>GSHMNARPLPAGLTASQQWTLLEWIHMAGHIETEGELKAFLDNILSQAPSDRIILVLGRLNNQNQIQRMEKVLNVSYPSDWLNQYSQENFAQHDPIMRIHLGQGPVIWEERFSRAKGSEEKRF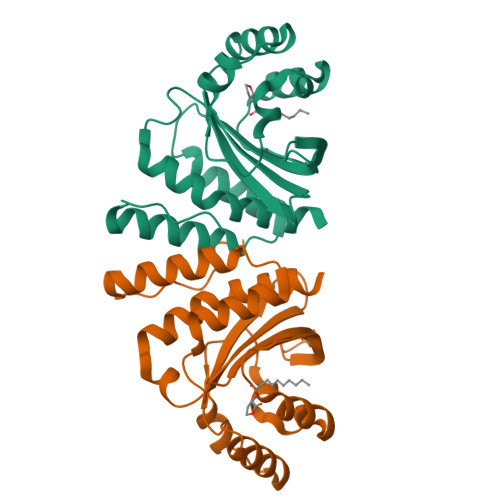IAEASSNGMGSGITFSAASDRNNVGSILSIGGKEPGRNAALVAMLNCLTPHLHQAAVRIAN[4x]> MVTSEQLLFLEAWRAVDRAYVDKSFNGQSWFKLRETYLKKEPMDRRAQTYDAIRKMLAVLD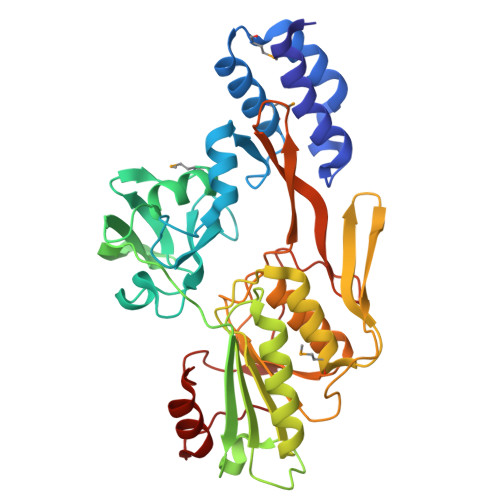DPFTRFLEPSRLAALRRGTAGSVTGVGLEITYDGGSGKDVVVLTPAPGGPAEKAGARAGDVIVTVDGTAVKGMSLYDVSDLLQGEADSQVEVVLHAPGAPSNTRTLQLTRQKVTINPVTFTTCSNVAAAALPPGAAKQQLGYVRLATFNSNTTAAAQQAFTELSKQGVAGLVLDIRNNGGGLFPAGVNVARMLVDRGDLVLIADSQGIRDIYSADGNSIDSATPLVVLVNRGTASASEVLAGALKDSKRGLIAGERTFGKGLIQTVVDLSDGSGVAVTVARYQTPAGVDINKIGVSPDVQLDPEVLPTDLEGVCRVLGSDAAPRLFG>MSK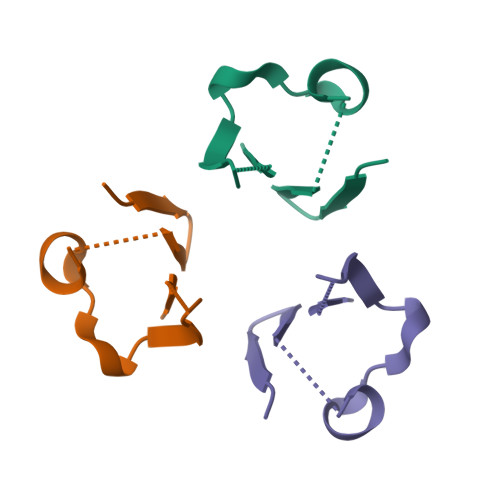VISTPDAPAAIGPYCQARLCDRTLYTSGIIGNDPHGGPNPETVEGQAELIMKSLDAMLKAAGYEKTDVVKCNCYLADIADFQKFNKIYADYFGDHKPCRCCIQAGKLPAGKLVELDAIAYK[4x]>[2x]MAHHHHHHMRKIYIAGPAVFNPDM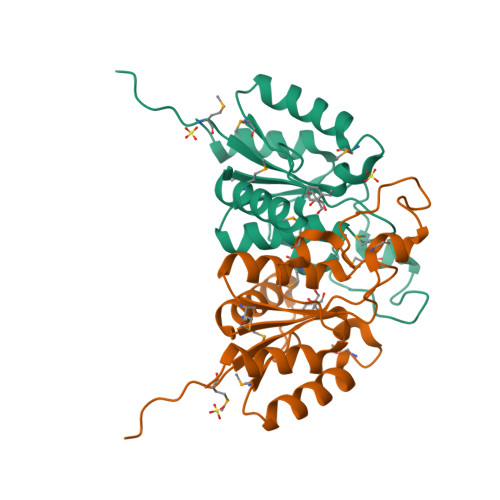GASYYNKVRELLKKENVMPLIPTDNEATEALDIRQKNIQMIKDCDAVIADLSPFRGHEPDCGTAFEVGCAAALNKMVLTFTSDRRNMREKYGSGVDKDNLRVEGFGLPFNLMLYDGVEVFDSFESAFKYFLANFPSK>[4x]KEAETQQKLANVVILATGGTIAGAGASAANSATYQAAKLGVDKLIAGVPELADIANVRGEQVMQIASESISNDDLLKLGKRVAELAESKDVDGIVITHGTDTLEETAFFLNLVEKTDKPIVVVGSMRPGTAMSADGMLNLYNAVAVASDKQSRGKGVLVTMNDEIQSGRDVSKAVNIKTEAFKSAWGPMGMVVEGKSYWFRLPAKRHTVNSEFDIKQISSLPQVDIAYGYGN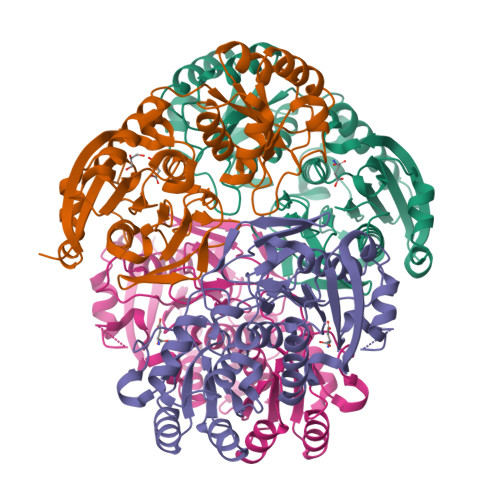VTDTAYKALAQNGAKALIHAGTGNGSVSSRVVPALQELRKNGVQIIRSSHVNQGGFVLRNAEQPDDKNDWVVAHDLNPQKARILAMVAMTKTQDSKELQRIFWEY> ASSLPPNALKPAFGPPDKVAAQKFKESLMATEKHAKDTSNMWVKISVWVALPAIALTAVNTYFVEKEHAEHREHLKHVPDSEWPRDYEFMNIR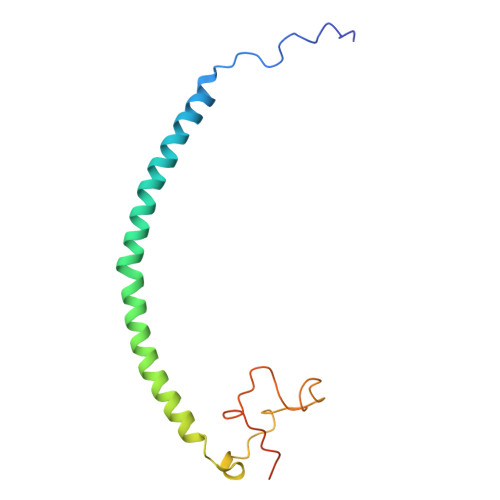SKPFFWGDGDKTLFWNPVVNRHIEHDDGARGSHHHHHH> TTSLTITEPDVDDDSTSDMEAFMAGVLVRYRKTLIEKTKYHLGYPFNLDLDYGPLAELQHFAINNLGDPFIESNYGVHSRQFEVGVLDWFARLWEIEQKEYWGYITNGGTEGNLHGILIGREVFPDGIFYTSRESHYSIFKAARMYRMECVKVGTLINGEIDCADFKAKLLSNKDKPAIINLNIGTTVKGAVDDIDLVIQTLEECGFSHDRFYIHCDGALFGFMMPFLNRGPKITFKKPIGSVSVSGHKFMGCPTPCGVQITRLEHINALSRNVEYLASRDATITGSRNGHSPIILWYALNRKGFKGFQKEVQKCLRNAHYLKDRLREAGISAMLNELSSTVVFERPLDEEFVRRWQLACEGNMAHVIVMPNVTIEKLDEFLNELVQKRANWYNDGKAGPPCLAPDIGSENCDCDLHKLEH

Ethylamine (EA), the precursor of theanine biosynthesis, is synthesized from alanine decarboxylation by alanine decarboxylase (AlaDC) in tea plants. In this study, we solved the X-ray crystal structures of AlaDC from Camellia sinensis (CsAlaDC) and SerDC from Arabidopsis thaliana (AtSerDC). CsAlaDC and AtSerDC are Group II PLP-dependent amino acid decarboxylases, which exhibit numerous structural features common to other amino acid decarboxylases. The overall structure of CsAlaDC or AtSerDC is homodimeric with two subunits exhibiting an asymmetrical arrangement.

Through optimization of crystallization conditions, we successfully determined the crystal structures of CsAlaDC, CsAlaDC-EA, and AtSerDC at resolutions of 2.50 Å, 2.60 Å, and 2.85 Å, respectively. The crystal structures of the CsAlaDC-EA complex and AtSerDC were obtained and further analyzed. In the former complex, PLP bound to Lys309 via a Schiff base linkage (internal aldimine form), and the pyridine moiety of PLP is positioned between the imidazole ring of His196 and the methyl group of Ala279 in a parallel orientation to the imidazole ring. The carboxylic group of Asp277 stabilizes the N1 of PLP by a salt bridge interaction, providing the latter with the strong electrophilicity necessary to stabilize carbon ion intermediates during enzymatic catalysis. The O3 forms hydrogen bonds with Thr247 and Lys309. Additionally, His308, Gly169, Thr170, Lys309, and Ser347*(‘*’ denotes the amino acids on adjacent subunits) establish a hydrogen bonding network with the phosphate group of PLP, consequently fortifying its attachment to the protein. Upon superimposing the active site residues of CsAlaDC apo and CsAlaDC-EA complex, it was observed that the hydroxyl group of Tyr336* in the CsAlaDC-EA complex exhibits a substantial 60 degree deviation along the Cα-Cβ bond. After the transaldimation of the internal aldimine within CsAlaDC, resulting in the release of the active-site residue Lys309, the pyridoxal-5-phosphate (PLP) amino acid external aldimine undergoes decarboxylation, leading to the removal of the α-carboxyl group as CO2. This process generates a quinonoid intermediate that is stabilized by the delocalization of paired electrons. The carbanion at Cα is subsequently protonated by the acidic p-hydroxyl group of Tyr336* located on the large loop, facilitated by its neighboring residue His196, which is situated on the small loop.> SPVAGQKYDYILVGGGTAACVLANRLSADGSKRVLVLEAGPDNTSRDVKIPAAITRLFRSPLDWNLFSELQEQLAERQIYMARGRLLGGSSATNATLYHRGAAGDYDAWGVEGWSSEDVLSWFVQAETNADFGPGAYHGSGGPMRVENPRYTNKQLHTAFFKAAEEVGLTPNSDFNDWSHDHAGYGTFQVMQDKGTRADMYRQYLKPVLGRRNLQVLTGAAVTKVNIDQAAGKAQALGVEFSTDGPTGERLSAELAPGGEVIMCAGAVHTPFLLKHSGVGPSAELKEFGIPVVSNLAGVGQNLQDQPACLTAAPVKEKYDGIAISDHIYNEKG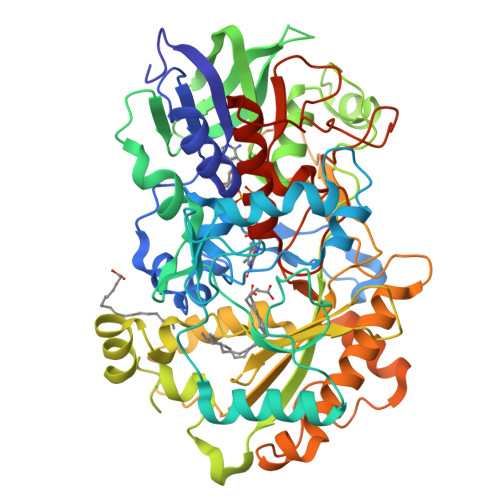QIRKRAIASYLLGGRGGLTSTGCDRGAFVRTAGQALPDLQVAFVPGMALDPDGVSTYVRFAKFQSQGLKWPSGITMQLIACRPQSTGSVGLKSADPFAPPKLSPGYLTDKDGADLATLRKGIHWARDVARSSALSEYLDGELFPGSGVVSDDQIDEYIRRSIHSSNAITGTCKMGNAGDSSSVVDNQLRVHGVEGLRVVDASVVPKIPGGQTGAPVVMIAERAAALLTGKATIGASAAAPATVAA> MPMISCDMRYGRTDEQKRALSAGLLRVISEATGEPRENIFF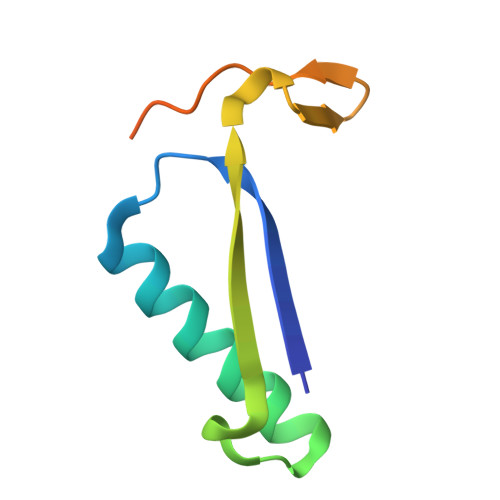VIREGSGINFVEHGEHLPDYVPGNANDKALIAKLK> MSSPLKNALVTAMLAGGALSSPTKQHVGIPVNASPEVGPGKYSFKQVRNPNYKFNGPLSVKKTYLKYGVPIPAWLEDAVQNSTSGLAERSTGSATTTPIDSLDDAYITPVQIGTPAQTLNLDFDTGSSDLWVFSSETTASEVDGQTIYTPSKSTTAKLLSGATWSISYGDGSSSSGDVYTDTVSVGGLTVTGQAVESAKKVSSSFTEDSTIDGLLGLAFSTLNTVSPTQQKTFFDNAKASLDSPVFTADLGYHAPGTYNFGFIDTTAYTGSITYTAVSTKQGFWEWTSTGYAVGSGTFKSTSIDGIADTGTTLLYLPATVVSAYWAQVSGAKSSSSVGGYVFPCSATLPSFTFGVGSARIVIPGDYIDFGPISTGSSSCFGGIQSSAGIGINIFGDVALKAAFVVFNGATTPTLGFASK

In this study, we used the aspartic protease endothiapepsin (EP), which serves as a model system for other aspartic proteases that play critical roles in several important diseases such as hypertension (renin), Alzheimer’s disease (β-secretase), malaria (plasmepsin IX/X) and HIV (HIV protease). EP has frequently been used to develop principles and fragment screening. Many fragment-based and inhibitor studies have found diverse ligand-binding modes in EP and, of these, ligand binding close to the catalytic centre of EP has been extensively studied. TL00150 binds to the active-site cleft of EP, in which 240 ligands were seen to bind.

A surprising fragment-binding discrepancy was observed between the cryo-cooled and physiological temperature structures, and multiple binding poses and their interplay with DMSO were captured. In addition, we found different binding modes for TL00150 between the S1 and S1′ positions in the EP structure that varied as a function of temperature and DMSO concentration. In comparison the 100 K structures only show a single stabilized protein state, which could have been introduced by the cryo-cooling procedure. However, at cryogenic temperatures protein plasticity can be limited due in part to the higher energy barrier that needs to be crossed to allow fragment binding when compared with room temperature. The difference in I/σ(I) and resolution range between the cryogenic and RT data in the highest resolution shell can be attributed to the use of different doses.>MDEQVIFTTNTSGTIASVHSFEQINLRQCSTQSRNSCVQVGNKYLFIAQAQKALINVYNLSGSFKRESVEQRLPLPEILKCLEVVENDGVQYDRIQGVNHNLPDFNLPYLLLGSTESGKLYIWELNSGILLNVKPMAHYQSITKIKSILNGKYIITSGNDSRVIIWQTVDLVSASNDDPKPLCILHDHTLPVTDFQVSSSQGKFLSCTDTKLFTVSQDATIRCYDLSLIGSKKKQKANENDVSIGKTPVLLATFTTPYSIKSIVLDPADRACYIGTAEGCFSLNLFYKLKGNAIVNLLQSAGVNTVQKGRVFSLVQRNSLTGGENEDLDALYAMGQLVCENVLNSNVSCLEISMDGTLLLIGDTEGKVSIAEIYSKQIIRTIQTLTTSQDSVGEVTNLLTNPYRLERGNLLFEGESKGKQPSNNNGHNFMKIPNLQRVIFDGKNKGHLHDIWYQIGEPEAETDPNLALPLNDFNAYLEQVKTQESIFSHIGKVSSNVKVIDNKIDATSSLDSNAAKDEEITELKTNIEALTHAYKELRDMHEKLYEEHQQMLDKQ[2x];>MSEEFIAVSTLARNLEIAKGNEFHTILATLRSPVYINEQLLKSELSFLVTKILKLIRSGNDFDLWKGCHTSVVTCAYNPLVLSTHGGQLLAAIYSRLEQKTGFYSSVISSSHGKQLFNTLISSVAIIIDLMKNKPTLSREALVPKLKAIIPTLITLSQYEPELVLPVLQRILKRNTTTFKPFTNKFRTVLINLIISDYASLGTKTQRLVCENFAYLHLLKIQVSDTSDDETQAHHKIYADSNWRTGLMSILSQFKPIIQLCGEILDFEQDNELYKLIKSLPVIDESNNKEEFLPSLKLDFNAPLTLWEIPQRLSLLADMLVAFISLPTPFPIRVPLGGINSLCEVLLGVSNKYLPLKKELRHDNELNGVINTILPQIQFQGIRLWEIMVSKYGKCGLSFFEGILSSIELFIPLKKKSNNEIDFNVVGSLKFEFATVFRLVNMILSHLGHQLNIISVISQLIEVALFLSHDKTLIDSLFKNRKSIMKQQTKTKQSKRSKSAEGAFSDIYTHPELFVCKNSMNWFNEINDFFITALNNWILPSTPHIQILKYSITQSLRLKERFGYIPESFVNLLRCEVLHPGSERVSILPIAISLLKNINDDMFELLCHPKVPVGMVYQLHKPLDLGEDGEVRDDINKKEVETNESSSNANTGLETLKALENLENVTIPEPKHEVPKVVDDTAIFKKRSVEEVIERESTSSHKKVKFVEETTVDNGEELIVKKAVSQTKEEEKPMEDSEDEEQEEFEIPAIELSDDEEEEEEEE[2x];> MTKSRKQKQKKQDFLRKKLKVGKPKEKARNATDTSFVSKTISIRNQHLDQNPHDLTKRLTLLKHHNINVRKE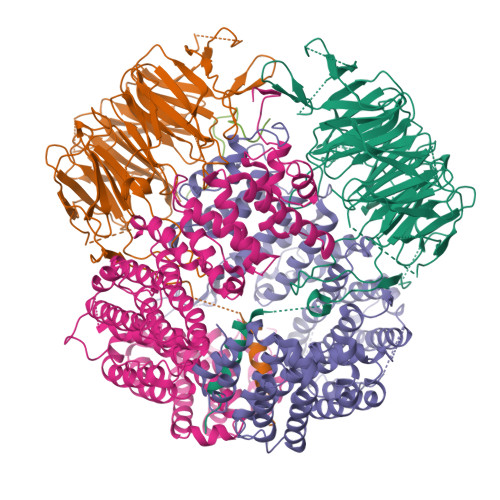TLTTFQKSIPSIIKSRLMTPLLTQSIPLICDESQQVRQGLIDLVDEIGSHDAEILKLHCNIFVLYINMAMTHIVTQIQADSTKFLSHLLKYCGDEVVRKSWVKLLNGVFGVLGWGQVGKNDSASIVQTKKRNAKYVTIHLNALYTLVEYGCQDERARSDGDTAETTEDSGTLRNPYLIPDYPQPFEHLKLFTRELKVQDATSSGVNATLLSLATQDIDTRKAVFIEQFLPIVRKKIEVIIKEGGECGKSANKLKTLLAKIFD The rhabdovirus matrix (M) protein is small (∼20–25 kDa) but plays a number of roles during the replication cycle of the virus. The M protein is an important structural component of rhabdovirus virions, forming a layer between the glycoprotein- (G-) containing outer membrane and the nucleocapsid core composed of the virus nucleoprotein (N), polymerase (L), phosphoprotein (P) and RNA genome. In addition to its structural roles, M has been implicated in controlling the balance between transcription and replication of the viral genome, in promoting budding, and in modulating host-cell transcription, -translation and -apoptosis. To further investigate the role of the N terminus and hydrophobic surface-exposed loop and to investigate the structural conservation of M across Rhabdoviridae, we solved the structures of full-length M from VSV serotype New Jersey (VSVNJ) and from the lyssavirus Lagos bat virus (LBV).

The structure of LBV M was solved by SeMet multi-wavelength anomalous dispersion phasing and refined to 2.75 Å resolution with residuals R/Rfree = 0.207/0.255. Residues 48–202 of LBV M form a globular domain with an overall fold that closely resembles those of VSVInd Mth and VSVNJ M, with 2.8 and 3.1 Å root-mean-squared deviation between 138 and 139 equivalent Cα positions, respectively, despite the aligned residues sharing less than 10% sequence identity. While the central α helix and back 5-stranded β sheet overlay very well, the loop between sheets β2 and β3 is much shorter in LBV M than in VSVNJ M and no stretch of helix is present between these sheets. Strikingly, in the structure of LBV M a stretch of peptide is again observed bound in a shallow hydrophobic groove formed by the β1–α1 and β2–β3 loops of the globular domain. W112 in the β2–β3 loop sits under residues 33–35, its indole nitrogen forming a hydrogen bond with the carbonyl oxygen of P34. Overall, these interactions bury 830 Å2 of surface area. The interaction with the most likely monomer, related by the crystallographic symmetry operator [1+x−y, 1−y, 1−z] (23 Å from E37 Cα to E48 Cα), generates linear polymers of non-covalently linked molecules in the crystal. The structure of LBV M therefore reveals both a novel 7th family of PRM-binding domain and defines the interaction of this domain with its cognate ligand. The polyproline-II helix conformation adopted by residues 32–36 of LBV M is entirely compatible with binding of this ‘late domain’ to the NEDD4 WW domain.

> MNFLRKIVKNCKDEEIPKPGTPSAPPDDDDLWMPPPEYVPLTQIKGKENVRNFCINGEIKICSPNGYSFRILRHILKSFDNVYSGNRRLIGVVKVVIGLVLSASPVPEGMNWVYKLRRTLIFQWAESHGPLEGEELEYSQEITWDDEAEFVSLQIRVSAKQCHIQGRLWCINMNSKACQLWADMGLKTQQSQEDENTSLLLE> GSGPPGPPGPPGPPGAR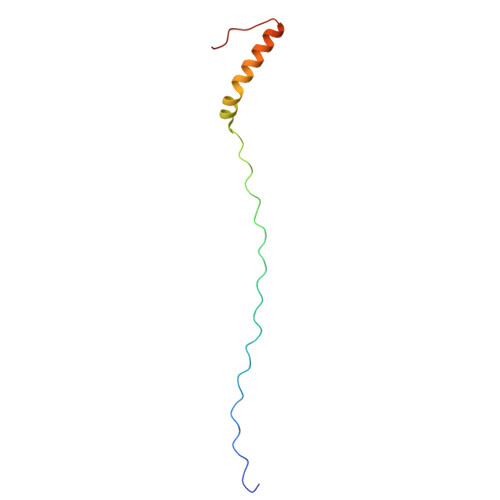GQAGVMGFPGPPGPPGPPGKEASEQRIRELCGGMISEQIAQLAAHLRKPLAPGSI>[2x]AALEPTDSGAPSAIVMFPVGEKPNPKGAAMKPVVFNHLIHEKKIDNCETCHHTGDPVSCSTCHTVEGKAEGNYITLDRAMHATNIAKRAKGNTPVSCVSCHE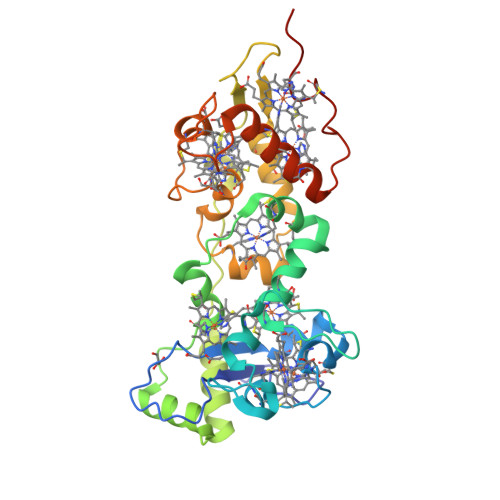QQTKERRECAGCHAIVTPKRDEAWCATCHNITPSMTPEQMQKGINGTLLPGDNEALAAETVLAQKTVEPVSPMLAPYKVVIDALADKYEPSNFTHRRHLTSLMERIKDDKLAQAFHNKPEILCATCHHRSPLSLTPPKCGSCHTKEIDKANPGRPNLMAAYHLQCMGCHKGMDVARPRDTDCTTCHKAAPKSAD> AQTNAAADWDVYCSQDESIPAKFISRLVTSKDQALEKTEINCSNGLVPITQEFGINMMLIQYTRNELLDSPGMCVFWGP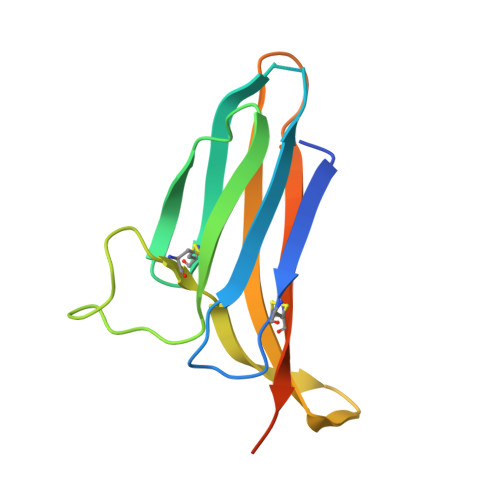YSVPKNDTVVLYTVTARLKWSEGPPTNLSIQCYMPKSPVAPKLEHHHHHH(6R,7R)-3-[(carbamoyloxy)methyl]-7-{[(2Z)-2-(furan-2-yl)-2-(methoxyimino)acetyl]amino}-8-oxo-5-thia-1-azabicyclo[4.2.0]oct-2-ene-2-carboxylic acid | C16 H16 N4 O8 S | 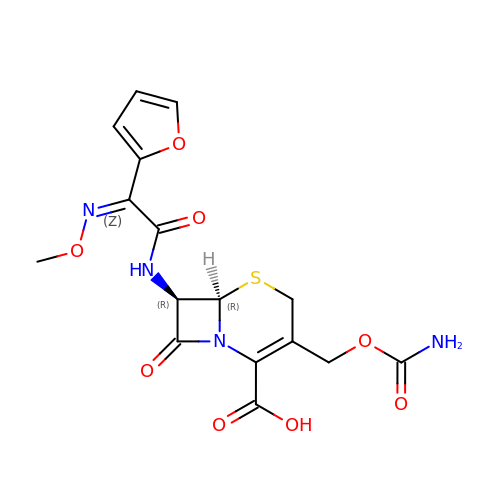JFPVXVDWJQMJEE-IZRZKJBUSA-N> TAPKSRNLFERNPNKELKPGENSPRQTPIFDPTVHWLFTTCGASGPHGPTQAQCNNAYQNSNLSVEVGSEGPLKGIQIWKVPATDTYSISGYGAAGGKGGKNTMMRSHGVSVLGIFNLEKDDMLYILVGQQGEDACPSTNQLIQKVCIGENNVIEEEIRVNRSVHEWAGGGGGGGGATYVFKMKDGVPVPLIIAAGGGGRAYGAKTDTFHPERLENNSSVLGLNGNSGAAGGGGGWNDNTSLLWAGKSLQEGATGGHSCPQAMKKWGWETRGGFGGGGGGCSSGGGGGGYIGGNAASNNDPEMDGEDGVSFISPLGIL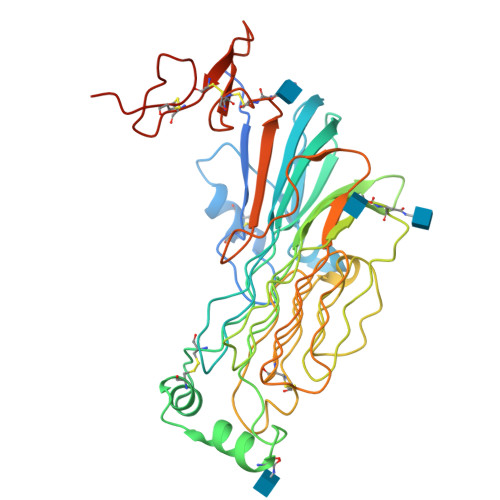YTPALKVMEGHGEVNIKHYLNCSHCEVDECHMDPESHKVICFCDHGTVLAEDGVSCIVSPTPEPHGTDEVD>MHEKTILVVDDEPRAREGMKRLLEKWASGKHRIITAANGQEALDILRQERVHVLLTDIRMPEITGLDVLEEMREKDDSPAVILISAYPDFDYAQKAISLGVLNYLLKPVKKSELFEA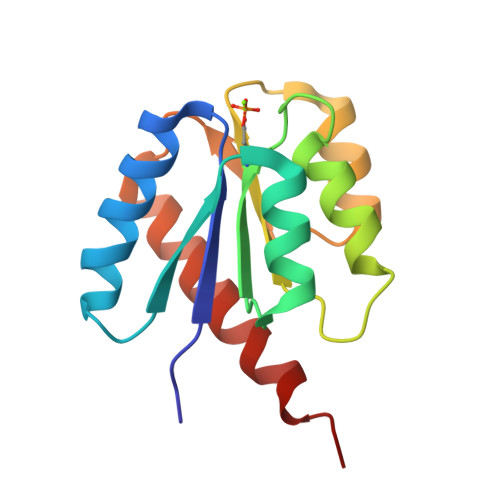VEKAIHVSEQKERERV[2x]> MSTNK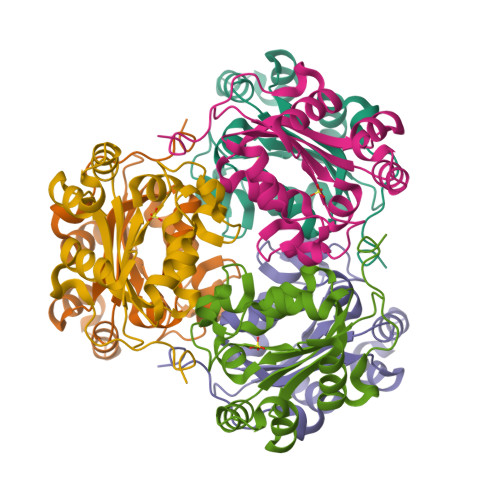VNKERTFLAVAPDGVARGLVGEIIARYEKKGFVLVGLKQLVPTKDLAESHYAEHKERPFFGGLVSFITSGPVVAMVFEGKGVVASARLMIGVTNPLASAPGSIRGDFGVDVGRNIIHGSDSVESANREIALWFKPEELLTEVKPNPNLYE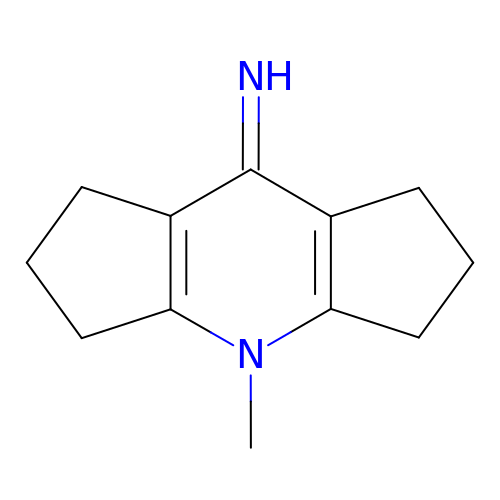4-methyl-2,3,4,5,6,7-hexahydrodicyclopenta[b,e]pyridin-8(1H)-imine | C12 H16 N2 | YOQONBCCIYETRK-UHFFFAOYSA-N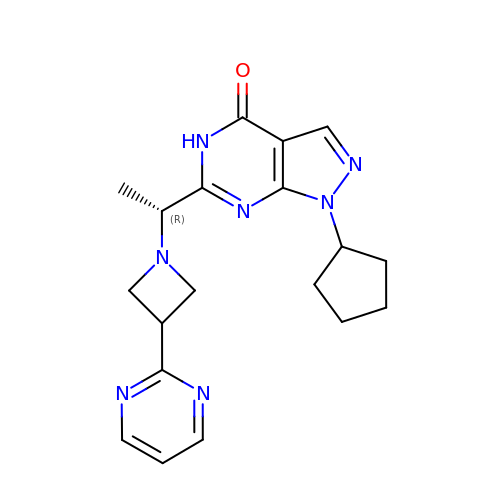1-cyclopentyl-6-{(1R)-1-[3-(pyrimidin-2-yl)azetidin-1-yl]ethyl}-1,5-dihydro-4H-pyrazolo[3,4-d]pyrimidin-4-one | C19 H23 N7 O | HJXAXXUTIBEZHT-GFCCVEGCSA-N> GSDDGAFGDIWAYMSEALTGAPGKIIACGMLFSVAYFGVVKPNLGLALVSALMMLVMANGEKIISSFL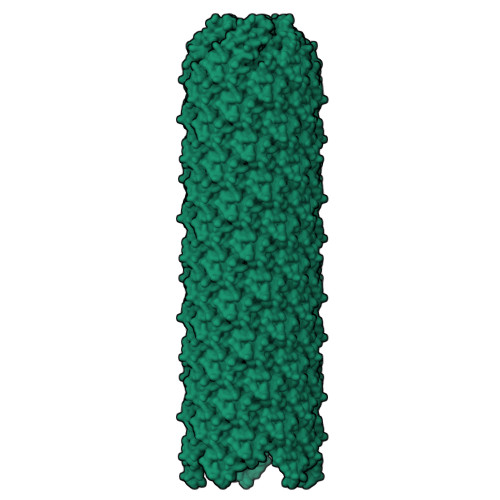NAGIPL> AAUUGAAAAAUCAAUAGAUUUAAACCUAGUGAAGAGCAUUUGAACAAUGUGCUAGGGUAGUAUGGGAUAAGUCGAUAACUAAAAUGAAUUGGGAUACUGAUUGAUUUUAGUGGUGGAUUUUACAGCAAUGUAAAAAGGACUAAUAGUAAAAGCUAUUAAUCGCAAAGUACUACGUGGAAUUUGUGCAGGUGUAAGGUACGAAACUUUCGAGUGUGACAAUAGACGCUCCAGUGGAGAAUAAUCUAAGUUAGGUGGAAGUGUGAGAAGCUUGGCAGACCUUAGAAAAC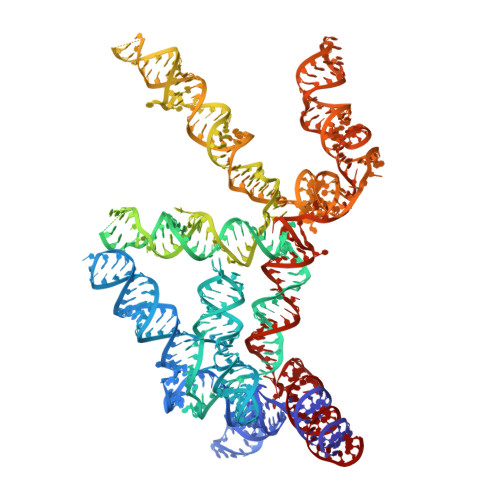UCAAACCAAGCGCUUUGCAGAGAAACUGAGAAAUCAGUGUUUAACGAAAGAAGUCGGUACGAGUAGCUUAAUGCAGCAAUUUAUUUACAGAUGACAAAUAAUAAAAAUGGGACUCUUAUGUAAAUGCUGAAUGUUCAAGUGAAAGUUAUUAGCCAGUAGAGCUAGAUCAUACAGAAAAAGCAAAGAGAAGCUAUUGGGUAGCGCCCGAUAGUUCAGCCUCUUUGGGUAUGUGACUGAAUAACACUGUAAACAAAGGAAGCAGGAAGAAAAGCCUAAAUCUGUUGAUUUUUGAG5-(5-formylthiophen-2-yl)uridine 5'-(trihydrogen diphosphate) | C14 H16 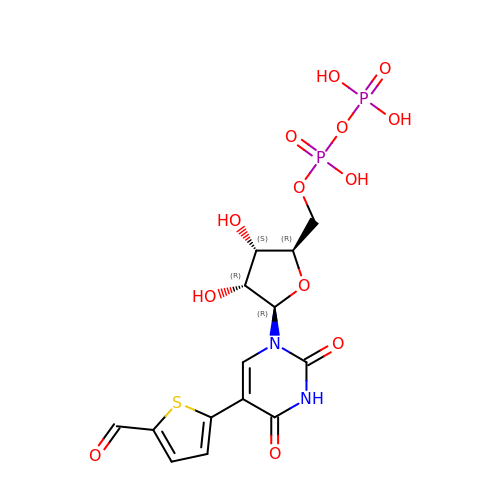N2 O13 P2 S | JAVHWQPALRUGBE-UORFTKCHSA-N> MSAEKLFTPLKVGAVTAPNRVFMAPLTRLRSIEPGDIPTPLMGEYYRQRASAGLIISEATQISAQAKGYAGAPGLHSPEQIAAWKKITAGVHAEDGRIAVQLWHTGRISHSSIQPGGQAPVSASALNANTRTSLRDENGNAIRVDTTTPRALELDEIPGIVNDFRQAVANAREAGFDLVELHSAHGYLLHQFLSPSSNQRTDQYGGSVENRARLVLEVVDAVCNEWSADRIGIRVSPIGTFQNVDNGPNEEADALYLIEELAKRGIAYLHMSETDLAGGKPYSEAFRQKVRERFHGVIIGAGAYTAEKAEDL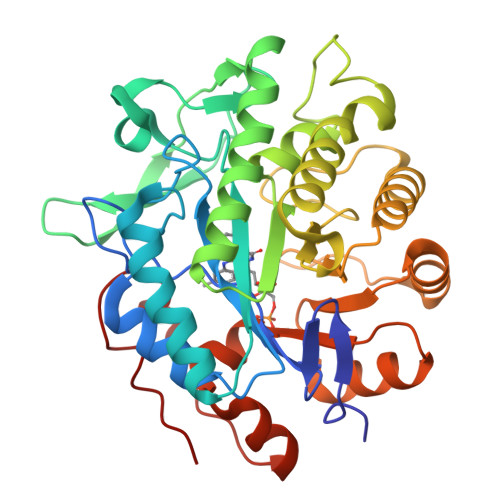IGKGLIDAVAFGRDYIANPDLVARLQKKAELNPQRPESFFGGGAEGYTDYPSL F-type ATP synthases are energy-converting membrane protein complexes that synthesize adenosine triphosphate (ATP) from ADP and inorganic phosphate. These universal enzymes function by using the energy stored in an electrochemical potential across the bioenergetic membrane by rotary catalysis. In mitochondria, F1Fo ATP synthase resides in the crista membrane where it is known to form dimers, which can further assemble into rows critical for inducing the membrane curvature and maintaining membrane potential and morphology. Here, we investigate the mechanism for the generation of the unique cristae in the Apicomplexa, using a combination of single-particle cryo-EM, cryo-ET and subtomogram averaging.

Masked refinements of the ATP synthase dimer resulted in maps of the membrane region, the OSCP/F1/c-ring complex, the rotor and the peripheral stalk, ranging in resolution from 2.8 to 3.5 Å, thus allowing de novo modelling of the respective regions. The attachment to F1 is mediated through OSCP, which adopts a fold conserved in prokaryotic and eukaryotic homologs. IF1 in our structure is bound exclusively to the α/β-interface facing the dimer interface, thereby locking it in the ADP-bound state (βDP). The N-terminal IF1 region that contacts the central stalk in the bovine complex25 is absent in our structure. Because central stalk rotation and conformational changes in the catalytic sites of F1 are interdependent, the sterically restrictive IF1 binding in T. gondii to only one of the three catalytic sites results in the trapping of the ATP synthase in a single rotational state in both the dimer and hexamer.

>[3x]MTIHSCLARRAVSVAASGARAFASGLGARAVAVGALQSARLLHTSSLRAAGAKISPSEMSRLLEERIAGWKTQTSTEEVGRVVSVGDGIARLFGLEGVQAGELVEFQNGMTGMALNLETDNVGVVIFGDDRSVLEGDSVKRTGRIVDVPIGPGLLGRVVDALGNPIDGKGPIPAKERRRVELKAPGIIPRKSVHEPMMTGLKCVDALVPVGRGQRELIIGDRQTGKTAVAVDAIINQKEINDSTDDESKKLYCIYVAVGQKRSTVAQIVKALEQRDAMKYTTVVAATASEAAPLQFLAPYSGCAMGEWFRDSGRHCVIIYDDLSKQATAYRQMSLLLRRPPGREAYPGDVFYLHSRLLERAAKMGDKSGGGSLTALPVIETQAGDVSAYIPTNVISITDGQIFLETELFYKGIRPAINVGLSVSRVGSAAQVKAMKQVAGTMKLELAQYREVAAFAQFGSDLDASTRQLLTRGTALTELLKQRQYSPMKNSVQVCVLYCGVKGYLDPLDPKEISRFESLFIDYINANHQDILKTIETEKELSEKTEAKLRAAVDEFVAMNEFKKK;>MASPALQTCWRNLARLSGAQVRPSHFGAFSLGSRMSPFSSLLGARASPIATGRAGLRFLSSAAPNPGKKPASAAPPAGTNHGRITQVIGAVVDVHFDEQLPPILNSLEVQGHTNRLVLEVAQHLGENTVRTIAMDATEGLVRGQKVVDTGAPIQVPVGVETLGRIMNVIGEPVDECGPVPAKKTYSIHRAAPLFADQSTEPGLLQTGIKVVDLLAPYAKGGKIGLFGGAGVGKTVLIMELINNVANKHGGFSVFAGVGERTREGNDLYHEMMTTGVIKRKKLEDGKFDFTGSKAALVYGQMNEPPGARARVALTALSVAEYFRDEQGQDVLLFIDNIYRFTQAGSEVSALLGRIPSAVGYQPTLATDLGQLQERITTTKKGSITSVQAVYVPADDLTDPAPATTFAHLDATTVLSRQIAELGIYPAVDPLDSTSRMLAPEIVGQEHYDTARATQKLLQDYKSLQDIIAILGMDELSEEDKLVVSRARKIQRFLSQPFTVAEVFTGKPGRFVELPETIKSAQTILRGECDDLPEMAFYMCGGLEEVRSKAVKMAQEAASGK[3x];> MALPLLASRRLFSSFVFRGQPSTLSSNLSLVRIRGLHGGSLSPPSATLPRAVQLFSSRIAFSTAAAEDSGASQTLEGRYASALFRVAKKKNQLEKVYGDLESVRNALKDSSEFRLFVDSPAVSVQQKLDVLRQLVNRYKFDPLTGNLLTTLVENKRLPMLARVADAFDAMYRKEKGEVKCLVTSAKPLSAQQQKEIVAALQNRAGTQARLIIDYAVSPQIMGGLVVRLGEQVLDFSVATRLDRLQSQLLAPL;>[10x]MFFSRLSLSALKAAPAREALPGLLSRQSFSSAGFSQFSSQKFFFSPSRNFSQSPLFQKHTPVHCNQRIASALVPTQQPAMTRQNPYAMQVGARYDAGVASLSAAIALMSVGGVAQGIGSLFAALVSGTARNPSIKEDLFTYTLIGMGFLEFLGIICVLMSAVLLYS;> MFARAFSRFASLAAPAPQRGWNAFVLPSRHFATAAGGANPFKNQLLLTLSSPSEAIYVRTPVRSVTVPGSEGAMTMTNGHSQTVARLKAGEIIVRKGETGDEVERFFLSDGFVLFKSPEDDSGCCTAEVLGVEVVPVSMLDKESAATALQELLQQGAGATDEWTKARTLLGQELLSSVIRAAP;> MWRSSGVSFTRYASEMAALLRQCLKEPYRTQAMQRNQIHLKETVYQQGQVLTRETFNDIKKAFEAAAKHAGEK;> MAGLASLSSVGALRGMRLVPAAHLLPLHSAFGQQTRNFGAGDLKIVAARMKSVKSIQKITKAMKMVAASKLRMDQRRLENGLPFATPVQKLVQRIPVDPKEKGTLAVLALSSDKGLCGGVNSFVAKQARIVIKENEMAGNAVQVYGVGDKIRSALQRTFGDRFKRIMTEVTRFPWNFGQACIIADRLMQDNPARLMVIYNHFKSAVAYDTLTLNVLTPTQAAQSAKEQLNTFEFEPEKTDVWKDLQDFYYACTVFGCMLDNIASEQSARMSAMDNASTNAGEMISSLTLRYNRARQAKITTELVEIISGANALE;> MSSPCCVAIRRVARTTLESGRRQVDSKSTDVSPFFTGTQQMSLPSAGMVTKIRNFSSVKFMDQKRSGEETVYFKKEDEALLRNLLANHPEYDPKYSVDHMNAEVGSIARDITLACQKHGMKDPSAAFMKDLISIFGAHGYAKNSK>[6x]GNLELALKALQILVNAAYVLAEIARDRGNEELLEKAARLAEEAARQAEEIARQARKEGNLELALKALQILVNAAYVLAEIARDRGNEELLEKAARLAEEAARQAEEIARQARKEGNLELALKALQILVNAAYVLAEIARDRGNEELLEKAARLAEEAARQAEEIARQARKEG

Circular tandem repeat proteins (‘cTRPs’) are de novo designed protein scaffolds (in this and prior studies, based on antiparallel two-helix bundles) that contain repeated protein sequences and structural motifs and form closed circular structures. While these cTRP constructs have many favorable properties, we have previously noted that their ability to self-assemble from smaller subunits is compromised by relatively limited contacts and small surface areas that are involved in packing between repeats and subunits. Based on those results, we hypothesized that a new generation of computationally designed cTRP proteins with increased repeat size (corresponding to longer secondary structural elements that increase both particle thickness and the number of buried contacts between repeats and protein subunits) would improve both the energetics and the stoichiometric control of self-association. In this study, we describe the de novo design of thick cTRPs (‘tcTRPs’) with repeats composed of longer helical bundles that form a new underlying repeat topology and demonstrate their solution and assembly behaviors, their structural features via X-ray crystallography and CryoEM, and their ability to be functionalized with additional folded protein domains.

To accomplish this, we generated and purified a construct that again contained only three repeats per subunit (termed ‘tcTRP93’). This construct was also expressed and purified at relatively high levels (yield ~5 mg per liter of culture) and eluted from a final SEC column at a volume corresponding to the same approximate mass as the full-length protein (left), indicating probable assembly into a higher-order trimeric species with 9 repeats total. The purified construct, also like the full-length protein, did not display significant unfolding behavior at 95° in a CD spectrum (right). The purified construct from the final SEC column was crystallized and its structure was determined at 3.2 Å resolution. This analysis confirmed a homotrimeric assembly that closely mirrored the dimensions, topology, and side-chain packing interactions found in the full-length tcTRP9 designed protein. In both cases, the assembled particles (‘tcTRP93-VHH3’) display three separate copies of the antiviral VHH domain in a trimeric organization extending from one face of the construct. The most active construct in our experiments (tcTRP93-VHH6813) displayed the lowest, sub-nanomolar values for both binding assays (KD and EC50 ~ 0.43 and 0.64 nM, respectively, and viral neutralization IC50 ~ 0.78 nM).>[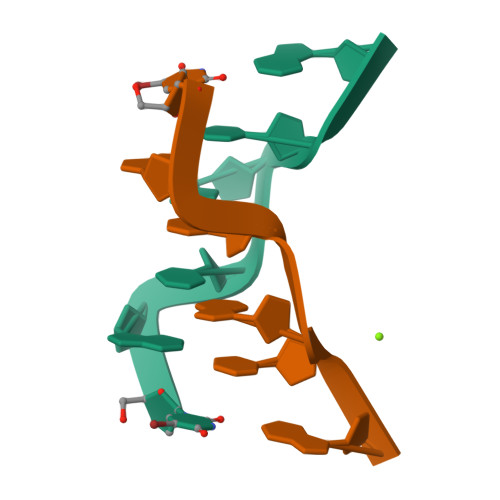2x]UGCGCG tetrahydro-2H-pyran-4-yl (3S,5'R)-2-oxo-1,2-dihydrospiro[indole-3,3'-pyrrolidine]-5'-carboxylate 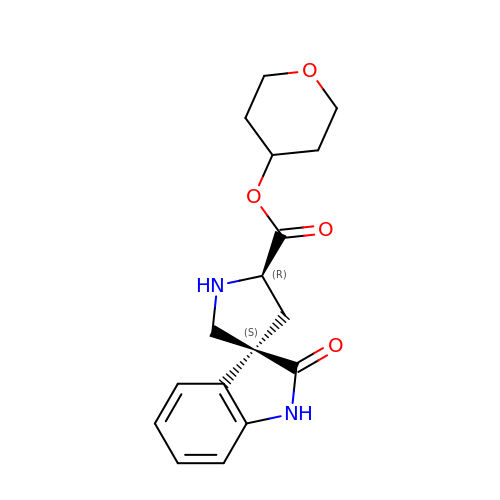| C17 H20 N2 O4 | HIOAPSYSJQPIRC-RHSMWYFYSA-N>LTAKKRPSVVYLHNAECTGCSESLLRTVDPYVDELILDVISMDYHETLMAGAGHAVEEALHEAIKGDFVCVIEGGIPMGDGGYWGKVGRRNMYDICAEVAPKAKAVIAIGTCATYGGVQAAKPNPTGTVGVNEALGKLGVKAINIAGCPPNPMNFVGTVVHLLTKGMPELDKQGRPVMFFGETVHDNCPRLKHFEAGEFATSFGSPEAKKGYCLYELGC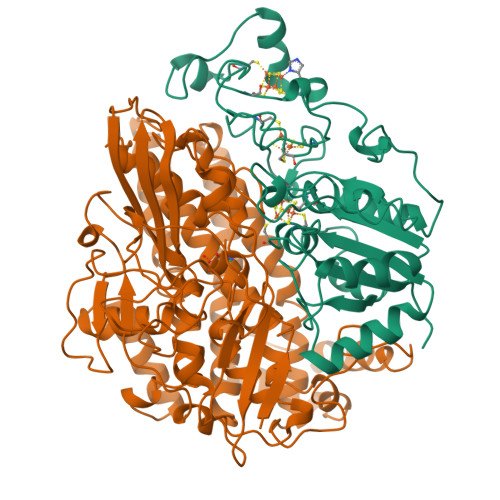KGPDTYNNCPKQLFNQVNWPVQAGHPCIACSEPNFWDLYSPFYSA[2x];>[2x]MSEMQGNKIVVDPITRIEGHLRIEVEVEGGKIKNAWSMSTLFRGLEMILKGRDPRDAQHFTQRACGVCTYVHALASVRAVDNCVGVKIPENATLMRNLTMGAQYMHDHLVHFYHLHALDWVNVANALNADPAKAARLANDLSPRKTTTESLKAVQAKVKALVESGQLGIFTNAYFLGGHPAYVLPAEVDLIATAHYLEALRVQVKAARAMAIFGAKNPHTQFTVVGGCTNYDSLRPERIAEFRKLYKEVREFIEQVYITDLLAVAGFYKNWAGIGKTSNFLTCGEFPTDEYDLNSRYTPQGVIWGNDLSKVDDFNPDLIEEHVKYSWYEGADAHHPYKGVTKPKWTEFHGEDRYSWMKAPRYKGEAFEVGPLASVLVAYAKKHEPTVKAVDLVLKTLGVGPEALFSTLGRTAARGIQCLTAAQEVEVWLDKLEANVKAGKDDLYTDWQYPTESQGVGFVNAPRGMLSHWIVQRGGKIENFQHVVPSTWNLGPRCAERKLSAVEQALIGTPIADPKRPVEILRTVHSYDPCIACGVH>[2x]MAFKLPNLPYAYDALEPYIDQRTMEFHHDKHHNTYVTKLNATVEGTELEHQSLADMIANLDKVPEAMRMSVRNNGGGHFNHS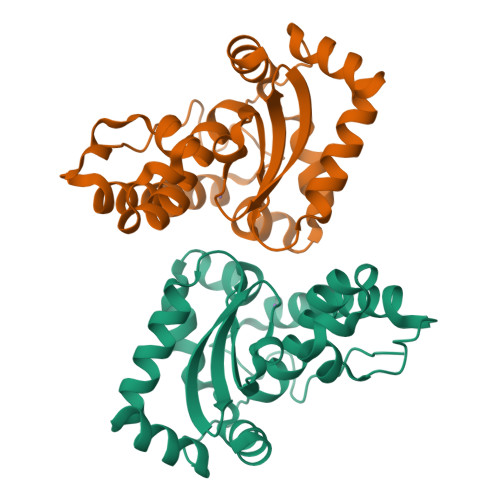LFWEILSPNSEEKGGVIDDIKAQWGTLDEFKNEFANKATTLFGSGWTWLVVNDGKLEIVTTPNQDNPLTEGKTPILGLDVWEHAYYLKYQNKRPDYMTAFWNIVNWKKVDELYQAAK> MVFLPLKWSLATMSFLLSSLLALLTVSTPSWCQSTEASPKRSDGTPFPWNKIRLPEYVIPVHYDLLIHAQLTTLTFWGTTKVEITASQPTSTIILHSHHLQISRATLRKGAGERLSEEPLQVLEHPRQEQIALLAPEPLLVGLPYTVVIHYAGQLSETFHGFYKSTYRTKEGELRILAS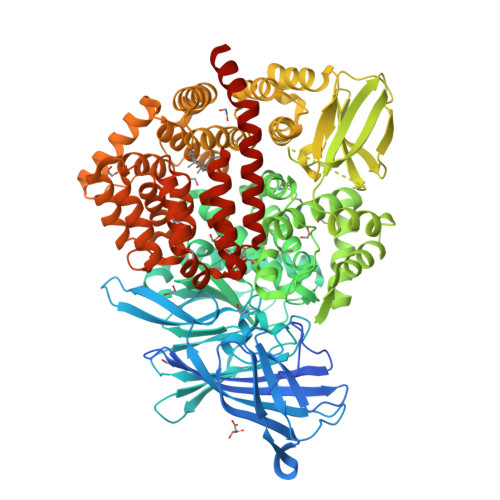TQFEPTAARMAFPCFDEPAFKASFSIKIRREPRHLAISNMPLVKSVTVAEGLIEDHFDVTVKMSTYLVAFIISDFESVSKITKSGVKVSVYAVPDKINQADYALDAAVTLLEFYEDYFSIPYPLPKQDLAAIPDFQSGAMENWGLTTYRESALLFDAEKSSASSKLGITMTVAHELAHQWFGNLVTMEWWNDLWLNEGFAKFMEFVSVSVTHPELKVGDYFFGKCFDAMEVDALQSSHPVSTPVENPAQIREMFDDVSYDKGACILNMLREYLSADAFKSGIVQYLQKHSYKNTKNEDLWDSMASIGSGGVDVKTMMNTWTLQKGFPLITITVRGRNVHMKQEHYMKGSDGAPDTGYLWHVPLTFITSKSDMVHRFLLKTKTDVLILPEEVEWIKFNVGMNGYYIVHYEDDGWDSLTGLLKGTHTAVSSNDRASLINNAFQLVSIGKLSIEKALDLSLYLKHETEIMPVFQGLNELIPMYKLMEKRDMNEVETQFKAFLIRLLRDLIDKQTWTDEGSVSERMLRSQLLLLACVHNYQPCVQRAEGYFRKWKESNGQLSLPVDVTLAVFAVGAQSTEGWDFLYSKYQFSLSSTEKSQIEFALCRTQNKEKLQWLLDESFKGDKIKTQEFPQILTLIGRNPVGYPLAWQFLRKNWNKLVQKFELGSSSIAHMVMGTTNQFSTRTRLEEVKGFFSSLKENGSQLRCVQQTIETIEENIGWMDKNFDKIRVWLQSEKLERMENLYFQ N-[6-(methylsulfonyl)-1,3-benzothiazol-2-yl]-2-[2-(1H-pyrrol-1-yl)-1,3-thiazol-4-yl]acetamide | C17 H14 N4 O3 S3 | 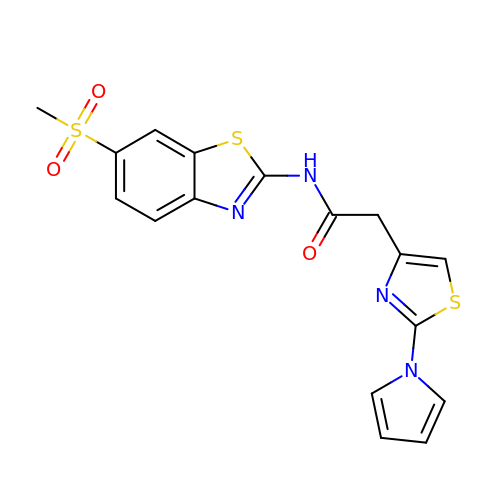KRKFVNMZGZWPHC-UHFFFAOYSA-N glaucine | C21 H25 N O4 | 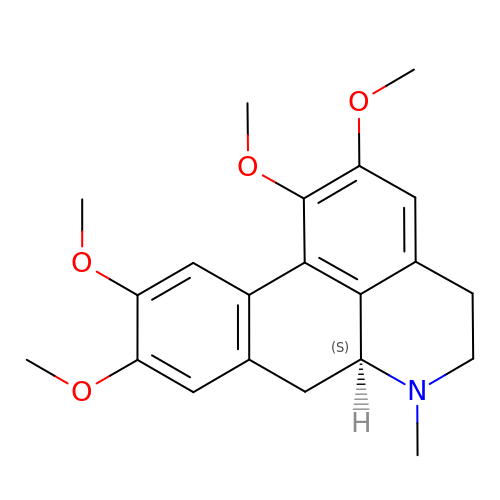RUZIUYOSRDWYQF-HNNXBMFYSA-N> SGDEADRTLF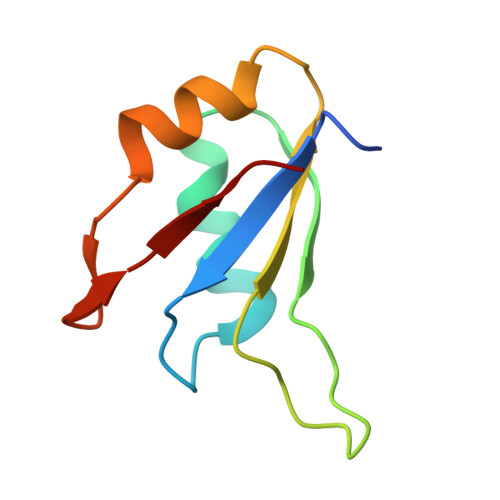VGNLETKVTEELLFELFHQAGPVIKVKIPKDKDGKPKQFAFVNFKHEVSVPYAMNLLNGIKLYGRPIKIQFRS Members of the virulence-associated protein (Vap) family from the pathogen Rhodococcus equi regulate virulence in an unknown manner. Rhodococcus equi is a Gram-positive facultative intracellular pathogen mainly of young foals, but also of other animal species and of human AIDS patients. VapB and VapA are normally associated with isolates from pigs and horses, respectively. The amino-acid sequence similarities between all Vap proteins according to ClustalW are typically in the 30–50% identity range, with the 78% identity score between VapA and VapB being particularly high.

Here, we present the crystal structure at 1.4 Å resolution of the 12 kDa C-terminal protease-resistant core of recombinantly produced VapB. Edman sequencing (Proteome Factory, Berlin) revealed that the resulting 12 kDa stable fragment started at amino acid Glu85. VapB crystallized in a condition containing 10 mM CoCl2 from a commercial screen. The anomalous signal originating from the S atom of the single methionine and two low-occupancy (∼25%) Co2+ ions was sufficient to solve the phase problem by SAD. Clear electron density is visible for residues Glu87–Val196 with some density for residues Gln86 and Ala197. VapB is an eight-stranded antiparallel β-barrel with a single helix. Unlike other eight- or ten-stranded β-barrels found in avidins, bacterial outer membrane proteins, fatty-acid-binding proteins and lysozyme inhibitors, Vaps do not have a next-neighbour arrangement but consist of two Greek-key motifs with strand order 41238567, suggesting an unusual or even unique topology. The connections between strands 1 and 2 and strands 7 and 8 (residues 99–101 and 181–184, respectively) display double conformations. It is conceivable that these turns/loops move to open a mainly hydrophobic binding site formed by the top of the VapB hydrophobic core. A function of VapB in binding some kind of ligand thus seems possible.

> EQEQQYDVHGNVISAAVYQKFHVYGPEDMVFDGDAGGLTIPGAGAFWGTLFTSDLQRLYKDTVSFQYNALGTYLNINFFDSSGGFLGHIQAGAVSAVVGVGGGSGSWHNWEVA PYK (EC 2.7.1.40) forms a tetramer that catalyzes transfer of phosphate from phosphoenolpyruvate (PEP) to ADP to form pyruvate and ATP. MtbPYK adopts a tetrameric architecture formed by identical subunits with three domains (A, B and C domains), similar to typical PYK structures. The catalytic site is located in the cleft between the A and B domains (lid domain), while the C domain harbours a canonical AMP allosteric site. The allosteric site binding for G6P (sugar monophosphate site) is adjacent to the AMP site and lies between the A and C domains.

In MtbPYK, the AMP phospho group is H-bonded to residues Thr374, Gln375, Ser376, Thr379 and AMP-loop residue Gly457, and forms a salt bridge with the side-chain of Arg351 in helix Cα1. The adenine-binding site for AMP is relatively hydrophobic and is composed of residues Phe373, Trp398 and Met425. These residues form stacking interactions with the adenine ring of AMP. Interestingly, the binding of Trp398 to AMP requires reorientation of the side chain of this residue to close up the AMP pocket. The fact that Trp398 is not highly conserved in other AMP-activated PYKs suggests a unique regulatory function in MtbPYK. AMP binding (purple) triggers nearly maximum Cα4 movement (~6°) but modest Cα1 movement. Thus, the displacements of helices Cα1 and Cα4 resulting in allosteric-site reshaping are not substantially regulated by rigid-body rotation, but instead are correlated with the presence of AMP and G6P. This unique ‘synergistic allostery’ suggests that the binding of either activator is able to initiate the movements of both Cα1 and Cα4 to a certain extent and consequently reshape the allosteric sites to favour binding of the other activator.

>GGHMTRRGKIVCTLGPATQRDDLVRALVEAGMDVARMNFSHGDYDDHKVAYERVRVASDATGRAVGVLADLQGPKIRLGRFASGATHWAEGETVRITVGACEGSHDRVSTTYKRLAQDAVAGDRVLVDDGKVALVVDAVEGDDVVCTVVEGGPVSDNKGISLPGMNVTAPALSEKDIEDLTFALNLGVDMVALSFVRSPADVELVHEVMDRIGRRVPVIAKLEKPEAIDNLEAIVLAFDAVMVARGDLGVELPLEEVPLVQKRAIQMARENAKPVIVATQMLDSMIENSRPTRAEASDVANAVLDGADALMLSGETSVGKYPLAAVRTMSRIICAVEENSTAAPPLTHIPRTKRGVISYAARDIGERLDAKALVAFTQSGDTVRRLARLHTPLPLLAFTAWPEVRSQLAMTWGTETFIVPKMQSTDGMIRQVDKSLLELARYKRGDLVVIVAGAPPGTVGSTNLIHVHRIGEDDV[4x]>MKAIPPKIWFETQLKGSGLDKKFQIDELIETQSSVRVFANKKYLPDTETINEALTKVTAVNVSGDKSGYFQNGLPFPNEAGYFEKIPVGHPELLSPIERLTGSKKIVSSHSLVTASGGYPLTNPLLPYRKPIRVSIFSLAGPSFENNYLHYRLFLLDSVQKIIDSPLFSHLHDGLPIQFDEAKKELGEYDTNKLMARIRLGFPYLARFSSGGFYPSFSKSNAIIFLSEAYFRYQLEDVSLLLASVNQTGKETGKAALLKATAVGMGFFAKIDCGYDIQHIIFPYYLRAYKKLLSEHKFPWIAKIEFPIFNEIQQEQFDSIFEDYDGPTKVYRST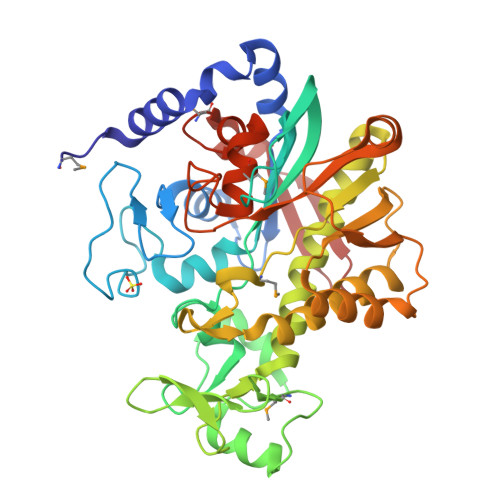RDVLEFREEEIEKYLPAAINPSDAFALTGNEWGYGSVESMIGNNSSIRFDQVHHMNPLILDPSHHVEAQINKDHGVELTVN[2x]>ARLGARPCGLRELEVRVSELGLGYASDETVLFRYCAGACEAAARVYDLGLRRLRQRRRLRRERVRAQPCCRPTAYEDE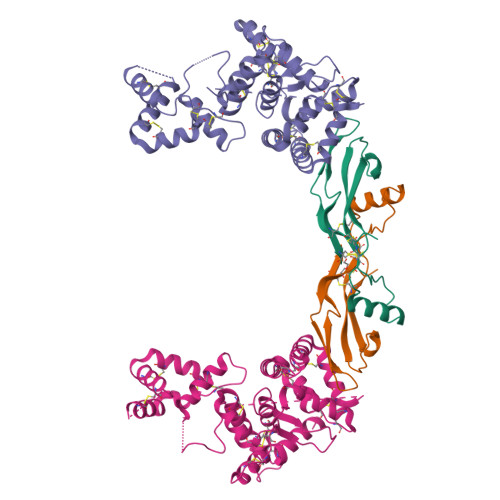VSFLDAHSRYHTVHELSARECACV[2x];>[2x]MILANVFCLFFFLDETLRSLASPSSLQGPELHGWRPPVDCVRANELCAAESNCSSRYRTLRQCLAGRDRNTMLANKECQAALEVLQESPLYDCRCKRGMKKELQCLQIYWSIHLGLTEGEEFYEASPYEPVTSRLSDIFRLASIFSGTGADPVVSAKSNHCLDAAKACNLNDNCKKLRSSYISICNREISPTERCNRRKCHKALRQFFDRVPSEYTYRMLFCSCQDQACAERRRQTILPSCSYEDKEKPNCLDLRGVCRTDHLCRSRLADFHANCRASYQTVTSCPADNYQACLGSYAGMIGFDMTPNYVDSSPTGIVVSPWCSCRGSGNMEEECEKFLRDFTENPCLRNAIQAFGNGTDVNVSPKGPSFQATQAPRVEKTPSLPDDLSDSTSLGTSVITTCTSVQEQGLKANNSKELSMCFTELTTNIIPGSNKVIKPNSGPSRARPSAALTVLSVL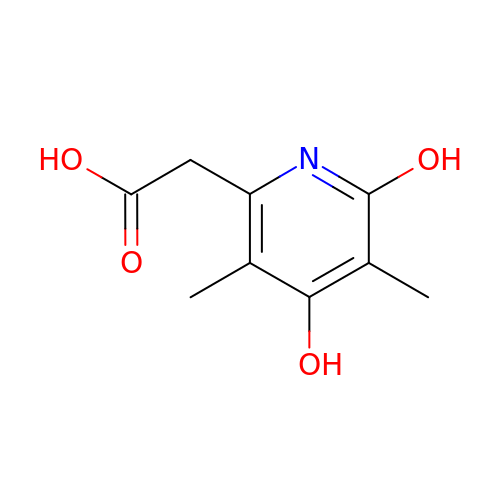(4,6-dihydroxy-3,5-dimethylpyridin-2-yl)acetic acid | C9 H11 N O4 | AVBVBQSPVBVXPJ-UHFFFAOYSA-N>[12x]MAQVQQLTPAQQAALRNQQAMAANLQARQIVLQQSYPVIQQVETQTFDPANRSVFDVTPANVGIVKGFLVKVTAAIKNNHATEAVALTDFGPANLVQRVIYYDPDNQRHTETSGWHLHFVNTAKQGAPFLSSMVTDSPIKYGDVMNVIDAPATIAAGATGELTMYYWVPLAYSETDLTGA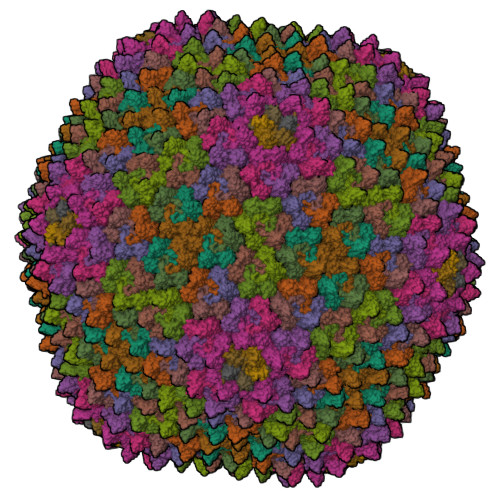VLANVPQSKQRLKLEFANNNTAFAAVGANPLEAIYQGAGAADCEFEEISYTVYQSYLDQLPVGQNGYILPLIDLSTLYNLENSAQAGLTPNVDFVVQYANLYRYLSTIAVFDNGGSFNAGTDINYLSQRTANFSDTRKLDPKTWAAQTRRRIATDFPKGVYYCDNRDKPIYTLQYGNVGFVVNPKTVNQNARLLMGYEYFTSRTELVNAGTISTT;> MALINPQFPYAGPVPIPGPAPTETMPLLNYRVEGRIAGIQQARQFMPFLQGPHREVAEQTYYAIGTGIQMGQTFNQPLINTQEG;> MDKKKLLYWVGGGLVLIIIWLWFRNRPAAQVASNWEGPPYMTYNQPQAGSVTLPVAGYTSPSLTLPNRNRSCGCNPAVSAAMAQGADLASKLTESISSQLNNYAESLNDYLASQAGV;>[3x]MANQQIGGSTVTYNGAIPMGGPVAINSVIEIAGTEVLVDLKLDYATGKISGVQTLYIDLRDFLGDVTVTMPDTGQRITARAGTQGYYPVLSTNLMKFIVSATIDGKFPMNFINFPIALGVWPSGIKGDKGDPGAPGPAGGTVVVEDSGASFGESLLDTTSEPGKILVKRISGGSGITVTDYGDEVEIEASGGGGGGGGVTDALSLMYSTSTGGPASIAANALTDFDLSGALTVNTVGTGLTKSAAGIQLAAGKSGLYQITMTVKNNTVTTGNYLLRVKYGSSDFVVACPASSLTAGGTISLLIYCDVLGVPSLDVLKFSLCNDGAALSNYIINITAAKIN;>MNVNNPNQMTVTPVYNGCDSGEGPQSVRGYFDAVAGENVKYDLTYLADTQGFTGVQCIYIDNAENDGAFEIDVEETGQRIKCPAGKQGYFPLLVPGRAKFVARHLGSGKKSVPLFFLNFTIAQGVW[2x]>[4x]MTANREAIDMARVAAGAAAAKLADDVVVIDVSGQLV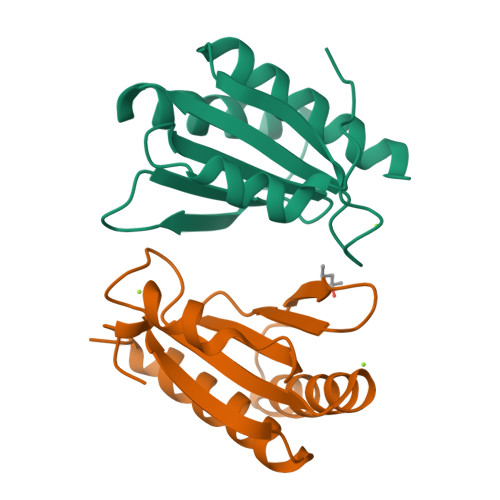ITDCFVIASGSNERQVNAIVDEVEEKMRQAGYRPARREGAREGRWTLLDYRDIVVHIQHQDDRNFAALDRLWGDCPVVPVDLSANSAGAQKLAAALEHHHHHH>MRGSHHHHHHGSKTIKIGIVGLGRLGKIHATNIATKIQHAKLQAATSVVPAELDWAKKELGVEEVFEDFDDMVQHADIDAVFIVSPSGFHLQQIESALNAGKHVFSEKPIGLDIEAIEHTQQVIAQHANLKFQLGFMRRFDDSYRYAKQLVDQGKIGDITLIRSYSIDPAAGMASFVKFATSANSGGLFLDMSIHDIDVIRWFTGKEIDKVWAIGLNRAYPVLDKAGELETGAALMQLEDKTMAILVAGRNAAHGYHV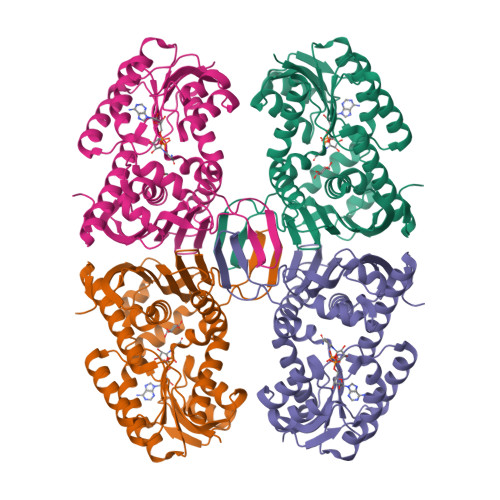ETEIIGTKGMLRIAQVPEKNLVTVMNEEGIIRPTSQNFPERFAQAFLSEEQAFVNSILNNQDVGITAEDGLQGTKAALALQEAFEKNDIVQVAS[4x]> MKDLVATTEMYLRTIYELEEEGVTPLRARIAERLEQSGPTVSQTVARMERDGLVVVASDRSLQMTPTGRTLATAVMRKHRLAERLLTDII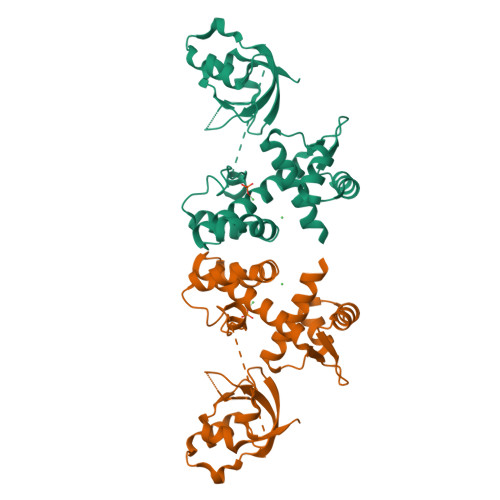GLDINKVHDEADRWEHVMSDEVERRLVKVLKDVSRSPFGNPIPGLDELGVGNSDAAAPGTRVIDAATSMPRKVRIVQINEIFQVETDQFTQLLDADIRVGSEVEIVDRDGHITLSHNGKDVELLDDLAHTIRIEEL>[2x]MSKAEKFYSLACYHAQLFSKDPNTKVAALVIDNNNNIAS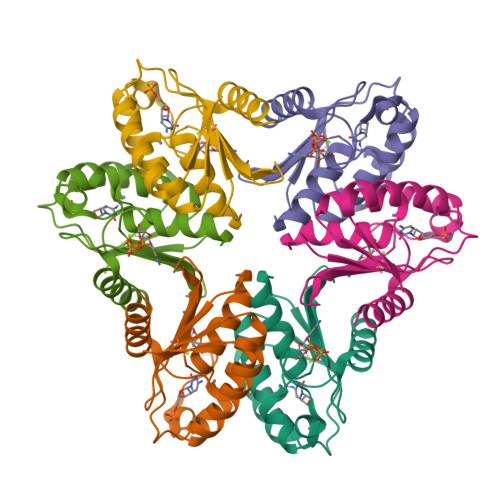VGYNGLPRGFEETSDRWEKPMKYNYVVHAQANAIATAARNGVRLDGCSIITTLFPCKECSKLIIQSGIRKVITSKPCKDSSWLESFSFSNEMFDECGIEVEYL> MDREQVVALQHQRFAAKKYDPNRRISQKDWEALVEVGRLAPSSIGLEPWKMLLLKNERMKEDLKPMAWGALFGLEGASHFVIYLARKGVTYDSDYVKKVMHEVKKRDYDTNSRFAQIIKNFQENDMKLNSERSLFDWASKQTYIQMANMMMAAAMLGIDSCPIEGYDQEKVEAYLEEKGYL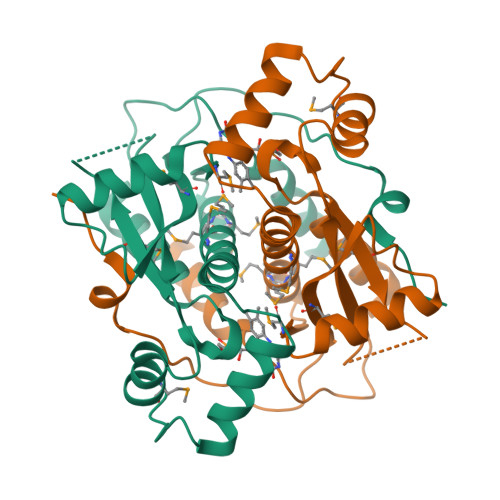NTAEFGVSVMACFGYRNQEITPKTRWKTEVIYEVIE> 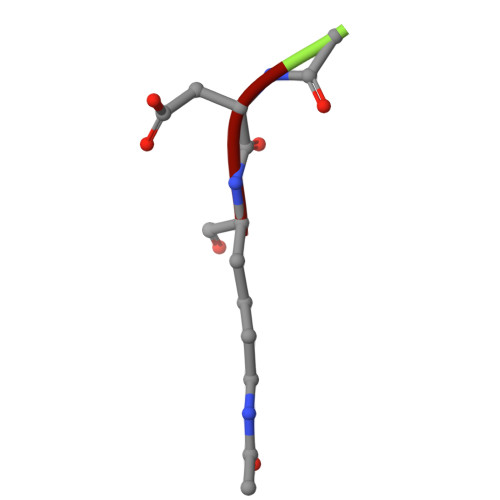SDK> MPITIGNGFLKSEILTNSPRNTKEAWWKVLWEKIKDFFFSTGKAKADRCLHEMLFAERAPTRERLTEIFFELKELACASQRDRFQVHNPHENDATIILRIMDQNEENELLRITQNTDTFSCEVMGNLYFLMKDRPDILKSHPQMTAMIKRRYSE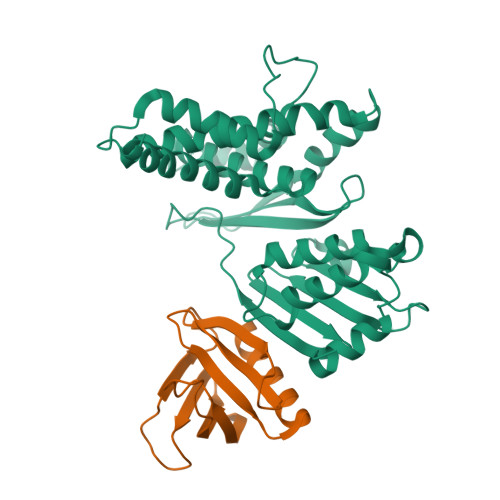IVDYPLPSTLCLNPAGAPILSVPLDNIEGYLYTELRKGHLDGWKAQEKATYLAAKIQSGIEKTTRILHHANISESTQQNAFLETMAMCGLKQLEIPPPHTHIPIEKMVKEVLLADKTFQAFLVTDPSTSQSMLAEIVEAISDQVFHAIFRIDPQAIQKMAEEQLTTLHVRSEQQSGCLCCFL;> TITKEGMLHYKAGTSYLGKEHWKTCFVVLSNGILYQYPDRTDVIPLLSVNMGGEQCGGCRRANTTDRPHAFQVILSDRPCLELSAESEAEMAEWMQHLCQAVSKG> MQDLEGKVAFVTGGGSGVALGQAKVLAEEAQMKVVIADIRQDHLDEAMGYFSQKNVAVHPVRLDLTDRAAYAAAVDEAEQVFGPVDLLCNTAGVSQFGPIEKATFDDWDWQMDVNVNGVINGVMTVMPRMIERGQGGHILITASMSAFVALPTTGIYCTTKYAVRGLAESLRVEMPKYNIGVSLLCPGGVNTNIHRSVEARPEKYGNTGYYGRDEAVFAGLKRVIEHGFDPVDLGRVVLDAVRNDRFWVLPYPEFAEGQKARDQEVIDAMMSYADHPDYA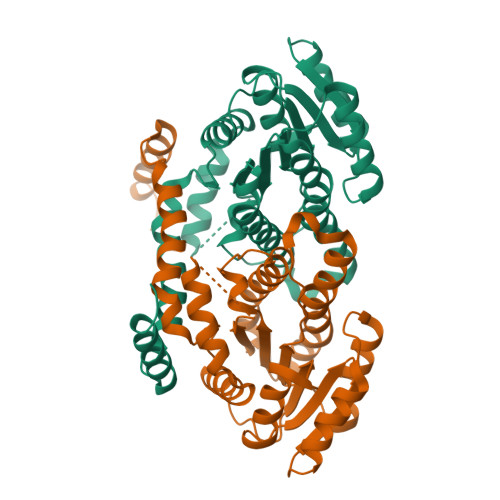RRMKIREQMKRDMPGSD> MPEISPHAPASADATRIAAIVAARQDIPGALLPILHEIQDTQGYIPDAAVPVIARALNLSRAEVHGVITFYHHFRQQPAGRHVVQVCRAEACQSVGAEALAEHAQRALGCGF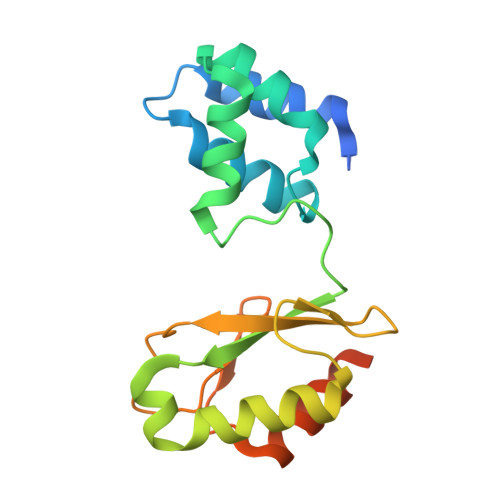HETTADGQVTLEPVYCLGQCACGPAVMVGEQLHGYVDARRFDALVRSLRESSAEKTTEAAEAQA>MAHHHHHHMAA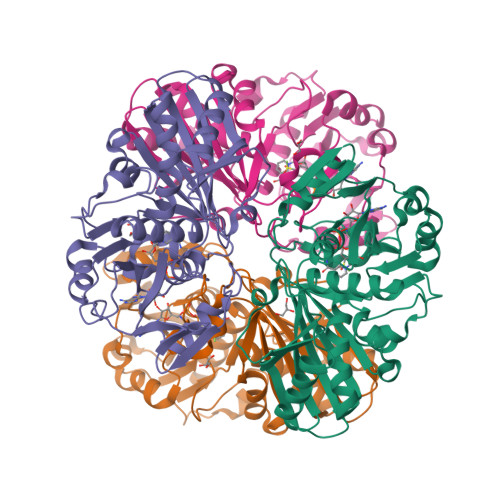TKLGINGFGRIGRLVFRAAFGRKDIEVVAINDPFMDLNHLCYLLKYDSVHGQFPCEVTHADGFLLIGEKKVSVFAEKDPSQIPWGKCQVDVVCESTGVFLTKELASSHLKGGAKKVIMSAPPKDDTPIYVMGINHHQYDTKQLIVSNASCTTNCLAPLAKVINDRFGIVEGLMTTVHASTANQLVVDGPSKGGKDWRAGRCALSNIIPASTGAAKAVGKVLPELNGKLTGVAFRVPIGTVSVVDLVCRLQKPAKYEEVALEIKKAAEGPLKGILGYTEDEVVSQDFVHDNRSSIFDMKAGLALNDNFFKLVSWYDNEWGYSNRVLDLAVHITTS[4x]2,5-dimethyl-4-sulfamoyl-furan-3-carboxylic acid | C7 H9 N O5 S | 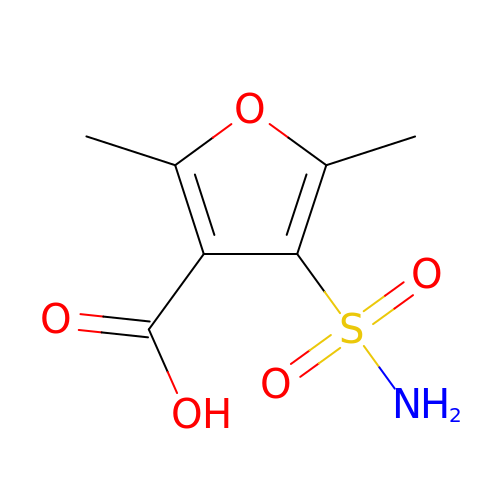YPWRJNLSEWKOGW-UHFFFAOYSA-N> GMKCNDKLAPFEVFDHVVNKKLSFRHVTMDDVDMLHSWMHEEHVIPYWKLNIPLVDYKKHLQTFLNDDHQTLMVGAINGVPMSYWESYWVKEDIIANYYPFEE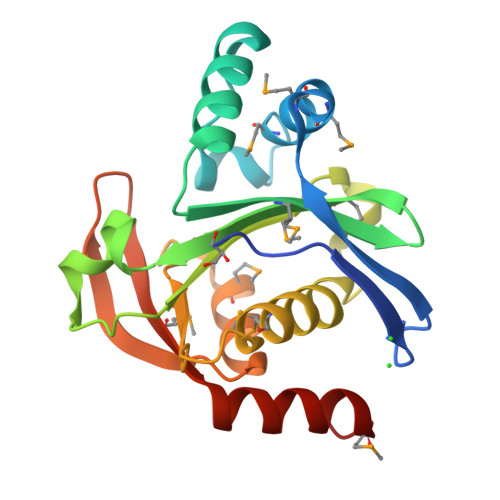HDQGIHLLIGPQEYLGQGLIYPLLLAIMQQKFQEPDTNTIVAEPDRRNKKMIHVFKKCGFQPVKEVELPDKIGLLMKCEQNVFEKRWSDWKMNKF> GPLGSMAKATTIKDAIRIFEERKSVVATEAEKVELHGMIPPIEKMDATLSTLKACKHLALSTNNIEKISSLSGMENLRILSLGRNLIKKIENLDAVADTLEE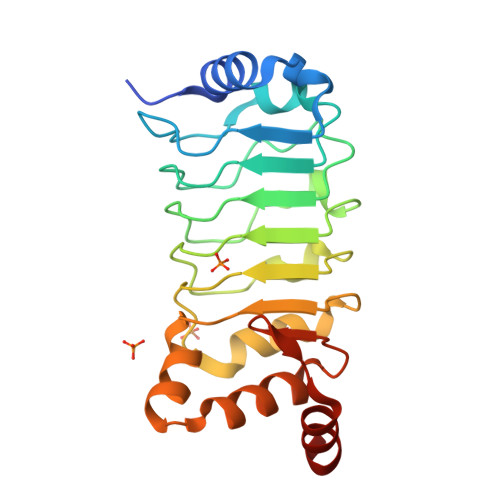LWISYNQIASLSGIEKLVNLRVLYMSNNKITNWGEIDKLAALDKLEDLLLAGNPLYNDYKENNATSEYRIEVVKRLPNLKKLDGMPVDVDEREQANVARGG>[9x]MKFLKNVLEEGSKLEEFNELELSPEDKELLEYLQQTKAKITVVGCGGAGNNTITRLKMEGIEGAKTVAINTDAQQLIRTKADKKILIGKKLTRGLGAGGNPKIGEEAAKESAEEIKAAIQDSDMVFITCGLGGGTGTGSAPVVAEISKKIGALTVAVVTLPFVMEGKVRMKNAMEGLERLKQHTDTLVVIPNEKLFEIVPNMPL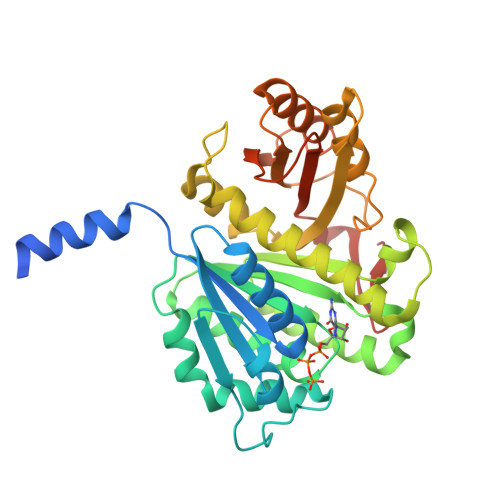KLAFKVADEVLINAVKGLVELITKDGLINVDFADVKAVMNNGGLAMIGIGESDSEKRAKEAVSMALNSPLLDVDIDGATGALIHVMGPEDLTLEEAREVVATVSSRLDPNATIIYGATIDENLENTVRVLLVITGVQSRIEFTDTGLKRKKLELTGIPKI> MIKIWVHIKNGSIYDITDIVDKVSWSGDYKSPSRTLEFSIIQSSFDNVFQQIDIPIASTVCFYVDEKELFRGMIINRSKDSSSNEISFVSKDMGFLLTQSEVSYNFKDKLVEDIAKQVFAENRLSVGIIAKTNVKYTKMFIGVNGYDTIMSAYTEASKKTKKKYMIEANLDKFNVIEKGTVTLSVMFEEGFNIINTTFSESMENVKNKVIVVDQYGSKISEKIDNEIFKEVNVIMQKVIQQQENQDVDIDSEFNGIEKSCSLKGYGDVSCITGRGVKVKDSYTKLVGLFYIDTDKHTWQNGEYQIELELNFQNLMDEKSAGQDEPKEESNLGGEDYAGGKEFTAEFTAYCPRKEEGGDTDCRKKKLDPSKKTCAAPMVGKYEQTYYTKEFLNKHPLLNYGDEIQVITGVSGRDGVYKVNDVGPAITIEKNGTYH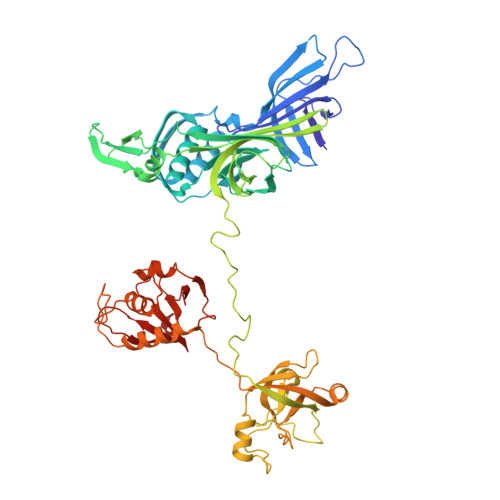IDILFGNVEEASKFGRRKGKIIIGGYSGNVSDKAKIVISEAKKHLGKPYKWGGNGPSSFDCSGLMVYCFKKVNVSLPRTSNQQSKKGKKVEQKNLQAGDLVFFHNPVSHVGLYIGNGEFLHAPQKGDVVKISKLSSRRDFNTARRVL>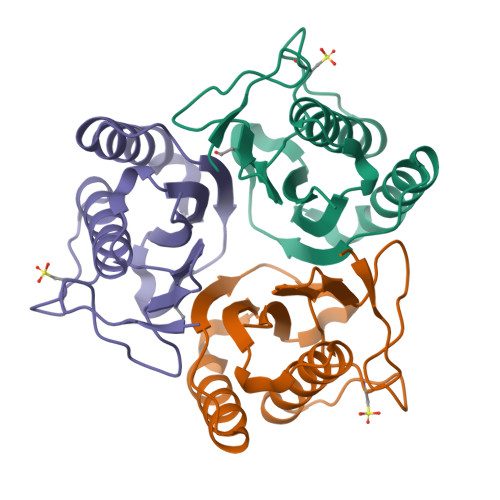[3x]MKKIIETQRAPGAIGPYVQGVDLGSMVFTSGQIPVCPQTGEIPADVQDQARLSLENVKAIVVAAGLSVGDIIKMTVFITDLNDFATINEVYKQFFDEHQATYPTRSCVQVARLPKDVKLEIEAIAVRSA F1Fo-ATP synthases are large, membrane-embedded macromolecular complexes that harness energy from the proton-motive force (pmf) and use it to synthesize ATP via a unique rotary mechanism. We solved the electron cryo-microscopy structure of the F1Fo–adenosine 5′-triphosphate (ATP) synthase from A. baumannii in three distinct conformational states. The A. baumannii ATP synthase has a subunit stoichiometry of α3β3γδεab2c10; its overall architecture resembles that of other bacterial and chloroplast ATP synthases. The rotating c-ring transfers torque to a central shaft comprising the ε- and γ-subunits, which protrude into the α3β3 hexamer, inducing conformational changes in the F1 nucleotide binding pockets, thus converting the rotary force into ATP synthesis.

State 1 was then used as a reference to build structures of the remaining two states. The central stalk is rotated by almost exactly 120o between each of the three conformational states suggesting common stable low-energy intermediate states in bacterial ATP synthases. Structural alignments of the γ-subunit between states revealed that the three states differ by almost exactly 120°. In F1, we observe the canonical “Walker-Boyer” state geometries in both the “open” conformation (βE, “empty”) and the “loose” conformation (βTP, with bound Mg–adenosine 5′-diphosphate). As in Bacillus PS3 (10), the third β-subunit (“tight” or βDP) is in a “forced open” conformation (denoted as βDP*), and we find only weak map features in this region, which we interpret as a loosely bound inorganic phosphate ion. The A. baumannii ε-subunit is similar to those seen in other bacteria, containing an extended C-terminal α helix. While the E. coli subunit ε bends here and protrudes “horizontally” between the αDP- and βTP-subunits, A. baumannii ε continues further upward into the F1 head, forming two more helical turns followed by a five-residue extension, which forms several additional interactions with the γ-, βTP-, and αDP-subunits. This may further stabilize subunit ε in the inhibitory “up” position, which blocks rotation in the hydrolysis direction, while still enabling ATP synthesis. The A. baumannii a-subunit contains an additional loop extension between aH4 and aH5. As the a-subunit loop insertion is conserved within the Acinetobacter family but is absent or structurally diverse in other bacteria and the mitochondrial ATP synthase, the unique a/c10 interface in A. baumannii represents a prime target for the development of highly specific inhibitors.

>[3x]MQQLNPSEISALIKQRIGDLDTSATAKNEGTIVMVSDGIVRIHGLADAMYGEMIEFDGGLFGMALNLEQDSVGAVVLGNYLSLQEGQKARCTGRVLEVPVGPELLGRVVDALGNPIDGKGPIDAKLTDAVEKVAPGVIWRQSVDQPVQTGYKSVDTMIPVGRGQRELIIGDRQTGKTAMAIDAIIAQKNSGIKCVYVAIGQKQSTIANVVRKLEETGAMAYTTVVAAAAADPAAMQYLAPYSGCTMGEYFRDRGEDALIIYDDLSKQAVAYRQISLLLRRPPGREAYPGDVFYLHSRLLERASRVSAEYVEKFTNGAVTGKTGSLTALPIIETQAGDVSAFVPTNVISITDGQIFLETSLFNAGIRPAVNAGISVSRVGGSAQTKIIKKLSGGIRTALAQYRELAAFAQFASDLDEATRKQLEHGQRVTELMKQKQYAPYSIADQAVSVYASNEGYMADVEVKKIVDFDAALIAYFRSEYAPLMKQIDETGDYNKDIEAAIKAGIESFKATQTY;>[3x]MSSGRIIQIIGAVIDVEFERTSVPKIYDALQVDGTETTLEVQQQLGDGVVRTIAMGSTEGLKRGLTVTSTNAPISVPVGTATLGRIMDVLGRPIDEAGPVATEERLPIHRQAPSYAEQAASTDLLETGIKVIDLLCPFAKGGKVGLFGGAGVGKTVNMMELINNIAKAHSGLSVFAGVGERTREGNDFYHEMKDSNVLDKVAMVYGQMNEPPGNRLRVALTGLTMAEYFRDEKDENGKGRDVLLFVDNIYRYTLAGTEVSALLGRMPSAVGYQPTLAEEMGVLQERITSTKSGSITSIQAVYVPADDLTDPSPATTFAHLDATVVLSRDIASSGIYPAIDPLDSTSRQLDPLVVGQEHYEIARAVQNVLQRYKELKDIIAILGMDELAEEDKLVVYRARKIQRFFSQPFHVAEVFTGAPGKLVPLKETIRGFKGLLAGEYDHIPEQAFYMVGGIDEVIAKAEKL;>MELTLGLVAIASAILIAFGALGTAIGFGLLGGRFLEAVARQPELAPQLQTRMFLIAGLLDAVPMIGVGIGLFFIFANPFVG[10x];> MAAEEHALTSTEYIKHHLTNMTYGKMPDGTWKLAETAEEAHSMGFTAIHLDSMGWSIGLGVIFCLLFWIVARAANAGVPTKFQSAIEMIIEFVDSSVRDTFHGKSRLIAPLALTIFVWIFLMNLMDLIPVDWIPQVAAFVGANVFGMDPHHVYFKIVPSTDPNITLGMSLSVFVLILFYSIREKGVGGFVGELALNPFNPSNPVAKALLIPVNLILELVTFLARPISLALRLFGNMYAGELIFILIALLPFWIQWALSVPWAIFHILVITLQAFIFMMLTIVYLSMASEKH;>[2x]MNINLTLIGQAIAFAFFVAFCMKFVWPPLINAISERQRKIADGLNAAEKAKADLADAQAQVKQELDAAKAQAAQLIEQANRRAAQLIEEARTQAAAEGERIRQQAKEAVDQEINSAREELRQQVAALAVTGAEKILNQQVDAEAHNAMLSQLAAKL;> MAELLTLARPYAKAAFAYASEQGATDNWSNALQVLSAAVQDEAFSAYLNRPELTPAEQVKLFAKVLGEDQSQAVSNFLTLLADNDRLVLLPEIAAEYEQLKSQNNNNVDVVIESAFPLTAEQEQLLKSALEKRFNSTVTVSVEVKPELIAGVVIRAGDQVIDDSALNKLEKMRTRLLA;> MATMQCDVVSVKESIYSGAVTMLIAKGAGGELGILPGHAPLVTLLQPGPIRVLLENGTEEIVYVSGGVLEVQPHVVTVLADTAIRADNLDEAAILEARKNAEQLLANQKSDLDSAAALAALAETAAQLETIRKIKNRAQ;> MANLKEIRAKVASIKSTQKITRAMQMVAASKMRRAQERMAQGRPYADNMRRVIAHLVQANPEYKHRYMVDRPVKRVGYIIVSSDRGLAGGLNINLFKKVVQHVKAQQEQSIEVQFALIGQKAVSFFKNYGGKVLGATTQIGDAPSLEQLTGSVQVMLDAFDKGELDRIYLVSNGFVNAMTQKPKVEQLVPLAPAEEGDDLNRTYGWDYIYEPEAEELLNGLLVRYIESMVYQGVIENVACEQSARMVAMKAATDNAGQLIKDLQLIYNKLRQAAITQEISEIVGGAAAV>[2x]EHPEFLKAGKEPGLQIWRVEKFDLVPVPTNLYGDFFTGDAYVILKTVQLRNGNLQYDLHYWLGNECSQDESGAAAIFTVQLDDYLNGRAVQHREVQGFESATFLGYFKSGLKYKKGGVASGFKHVVPNEVVVQR

Plasma gelsolin (pGSN) is the most abundant actin regulating protein in our plasma, and it’s major function is to scavenge F-actin released from the damaged or dying cells, thereby protecting microvasculature of our circulatory system. Bonsai gelsolin or fragment 28–161 of gelsolin represents a single domain of gelsolin family of proteins with slight tail or portion of g1-g2 linker of gelsolin which allows it to bind actin. For this step, extension of the tail is necessary which is achieved upon binding to Ca2+ ions or exposure to low pH. Detailed analysis brought forth that 28–161 has an inherent tendency to self-associate at temperatures around 30–45 °C and the association behavior is influenced by Ca2+ ions present in the buffer.

Of the different conditions tried, we could obtain diffractable crystals only at 18 °C and in the presence of Ca2+ ions. Any case, our crystal structure showed two Ca2+ ions bound to each chain of 28–161 and the G1 domains were arranged next to each other with few interactions stabilizing the interfacial contact. Each chain showed the typical gelsolin domain architecture of five β-sheets sandwiched between the two α-helices, with long helix running parallel to the β-sheets whereas the small helix was perpendicular to the β-sheets. Importantly, during refinement, we could not identify any electron density corresponding to the g1-g2 linker, possibly due to inherent flexibility across these residues. In our crystal structure, four Ca2+ ions were present in the entire assembly, two bound to each monomer, including both Type I (G65, E97, V145) and Type II (D109, G114, A116) Ca2+ binding sites. The interaction analysis revealed that the dimer is stabilized by one classical hydrogen bond between K150 → Y87, a salt bridge between H29 → E21 and numerous weak non-bonded interactions. Alignment of Cα trace of one chain in our crystal structure with same residues in the crystal structure of Ca2+-activated N-terminal half bound to actin provided an RMSD value of 0.45 Å. This information support that Ca2+ ions are sufficient to induce changes in G1 domain to bind actin and no additional significant changes happens post-binding to actin. Comparison of the two states of dimer of 28–161, one seen from our crystal structure bound to Ca2+ ions and other model fitted inside SAXS data based envelope to represent Ca2+-free dimer state showed that the difference lies in the relative orientation of the g1-g2 linker. Of particular interest is the residue Ala146 which acts as a fulcrum of this differential positioning with almost 180° flip of the tail region after it.> RPKLSEEQQHIIAILLDAHHKTYDPTYADFRDFRPPVRMDGSTGSVTLDLSPLSMLPHLADLVSYSIQKVIGFAKMIPGFRDLTSDDQIVLLKSSAIEVIMLRSNQSFTMDDMSWDCGSQDYKYDVTDVSKAGHTLELIEPLIKFQVGLKKLNLHEEEHVLLMAICIVSPDRPGVQDAKLVEAIQDRLSNTLQTYIRCRHPPPGSHQLYAKMIQKLADLRSLNEEHSKQYRSLSFQPENSMK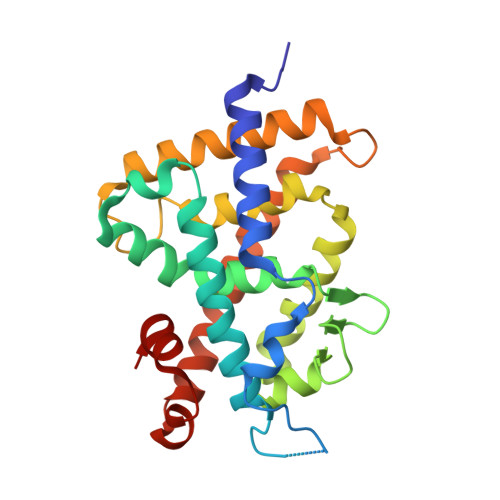LTPLVLEVFGN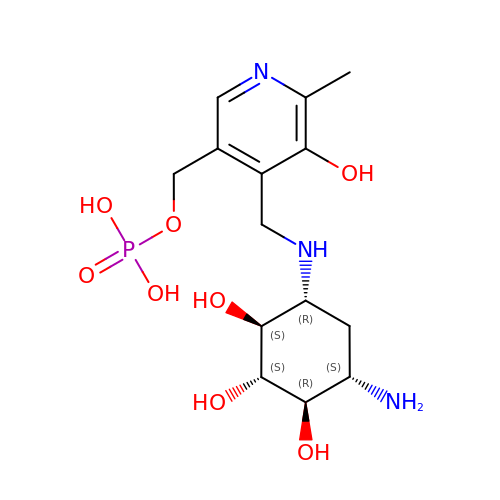[4-({[(1R,2S,3S,4R,5S)-5-amino-2,3,4-trihydroxycyclohexyl]amino}methyl)-5-hydroxy-6-methylpyridin-3-yl]methyl dihydrogen phosphate | C14 H24 N3 O8 P | QHLVFXGQUJCQEL-MYALOSSISA-N>[2x]GNDGGSDWVGKWQLREYQYPDGKVQKVDSIFYGFQKGSFLAYCMNKSGSYEGFY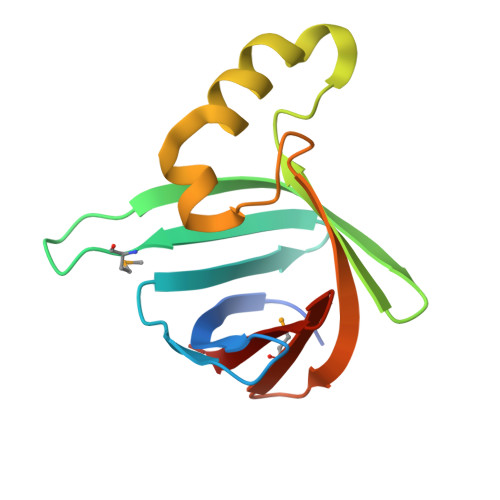GYYKLKDDEISITLWPDNSSGNEAAHEELVNSASYKNFFGWGDTGERTFKVEELTDKKMRLNYEGTKYVFRKY>GCCGAGCAGCA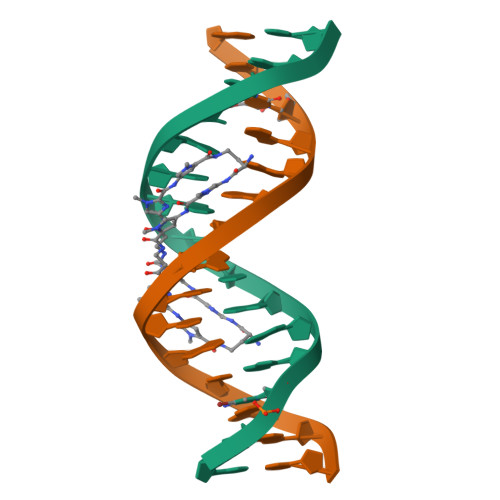CGGC[4x]>[2x]GDELYRQSLEIISRYLREQATGAKDTKPMGRSGATSRKALETLRRVGDGVQRNHETAFQGMLRKLDIKNEDDVKSLSRVMIHVFSDG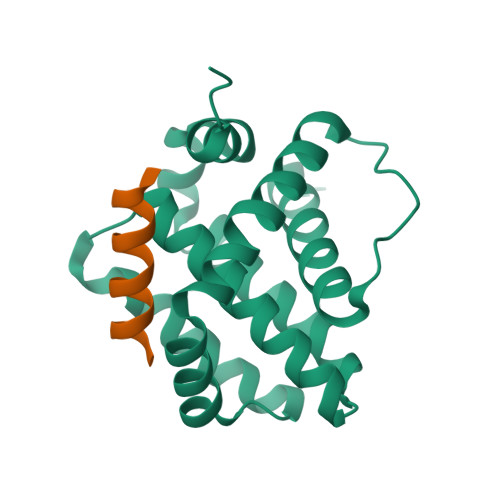VTNWGRIVTLISFGAFVAKHLKTINQESCIEPLAESITDVLVRTKRDWLVKQRGWDGFVEFFHVEDLEGG;>XALETLRRVGDGVQRNHX[2x]> MVIATIQAEDHSQQSGTQQETTT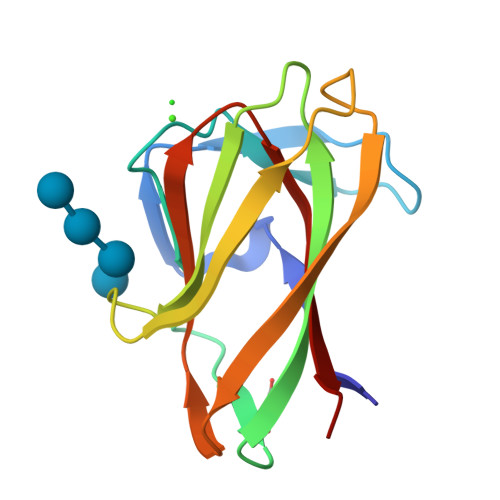DTGGGKNVGYIDAGDWLSYAGTPVNIPSSGSYLIEYRVASQNGGGSLTFEEAGGAPVHGTIAIPATGGWQTWTTIQHTVNLSAGSHQFGIKANAGGWNLNWIRINKTH C-terminal Src kinase (Csk) and Csk-homologous kinase (Chk) are members of the CSK family of protein tyrosine kinases. These proteins suppress the activity of Src family kinases (SFKs) by selectively phosphorylating the conserved C-terminal tail regulatory tyrosine. Csk and Chk both contain SH3, SH2, and kinase domains, which are separated by the SH3–SH2 and SH2-kinase linkers. The Csk SH2 domain is crucial in stabilizing the kinase domain in the active conformation.

Crystal structures of both oxidized SH2 and C122S SH2 were solved and refined. Intrinsic fluorescence of oxidized and reduced form of L-SH2 domain, as well as that of the cysteine mutants C122S and C164S L-SH2, was measured to examine the role of the disulfide bond in the stability of the Csk SH2 domain. U,W0 of the reduced, oxidized, C122S and C164S L-SH2 are 27.5 ± 0.7, 42.2 ± 1.6, 29.4 ± 0.9, and 26.3 ± 0.9 kJ/mol, respectively. All of the three forms of L-SH2 without disulfide bond were greatly destabilized compared with L-SH2 containing disulfide bonds with free energy value reductions ranging from 12.8 to 15.9 kJ/mol. The S–S distance of the disulfide bond was 2.0 Å, whereas the O–S distance in the C122S mutant was 3.7 Å. X-ray crystallography data were also consistent with the NMR observation, in which most of the changes in chemical shift took place in the residues close to C122, and this area was likely to undergo greater structural change than in the C164 residue area. Although the side chain direction of C122S residue was slightly different, the overall backbone position was nearly identical to that of the oxidized form and superimposes on the structures of Cα atoms that display a root-mean-square deviation of 0.19 Å. The overall backbone position of C122S and the oxidized form in the crystal structure is nearly identical, suggesting that the disulfide stability results from reduction of entropy of the unfolded state. Comparison of the crystal structure of the different forms of SH2 suggests that only minor structural changes resulted from the disulfide bond.

> AGTKLSLMPWFHGKITREQAERLLYPPETGLFLVRESTNYPGDYTLCVSSDGKVEHYRIMYHASKLSIDEEVYFENLMQLVEHYTSDADGLCTRLIKPKVMEGTVA>[2x]AGLSPEEQIETRQAGYEFMG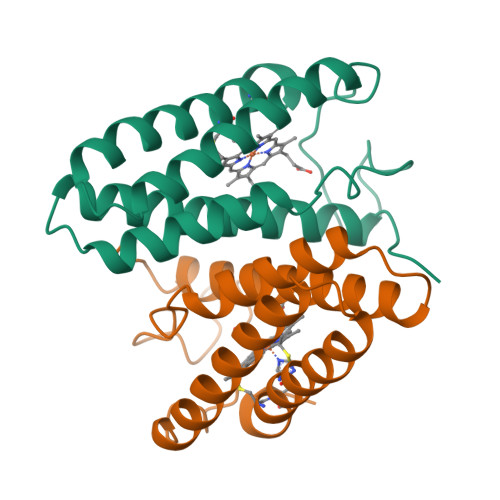WNMGKIKANLEGEYNAAQVEAAANVIAAIANSGMGALYGPGTDKNVGDVKTRVKPEFFQNMEDVGKIAREFVGAANTLAEVAATGEAEAVKTAFGDVGAACKSCHEKYRAK N,N'-OCTANE-1,8-DIYLBIS(2,3-DIHYDROXYBENZAMIDE) 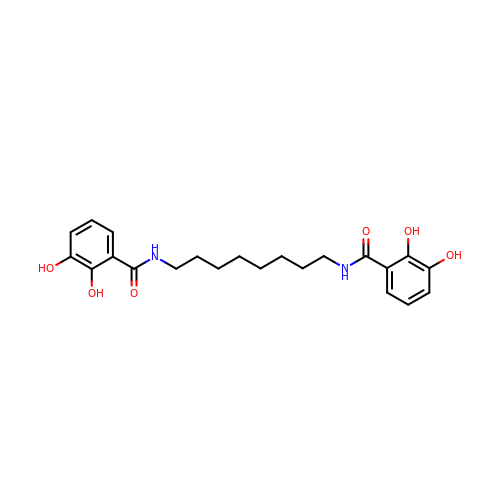| C22 H28 N2 O6 | DREKRZFIOMALFJ-UHFFFAOYSA-N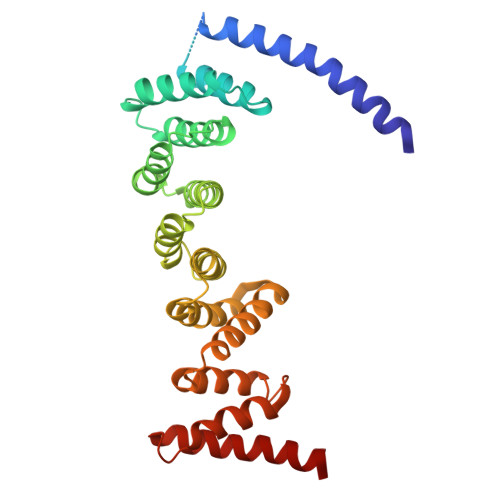> DNLRHFVQDYAVRALIPYIEHLVAILAEGVTNKKGVSKSLLSATKRWFVTSKPGAGANNQNAVIYTNESAELQTRKLGDLYFMFGHYNLAFQSYHQAKRDFNADSAWQYYAGALEMAALSAFMLGTAQRKTYDYMEDAIVCYLTVCKLQQFATRATLLSMECLKTARLYSEVAKQLIRMTNEESDLRSALLLEQAAYCFLVTQPPMHRKYAFHIVLAGNRYSRAGQRKHAYRCYRQAYQVFQKREWSLAEDHIQYTVAKQAYMLKQLEEASRSFAHLLRPGSLQSAQQQTSFLKEYIQTQNELVKRS>MRNQELARIFEEIGLMSEFLGDNPFRVRAYHQAARTLYDLDTPIEEIAEKGKEALMELPGVGPDLAEKILEFLRTGKVRKHEELSRKVPRGVLEVMEVPGVGPKTARLLYEGLGIDSLEKLKAALDRGDLTRLKGFGPKRAERIREGLALAQAAGKRRPLGAVLSLARSLLEAIRALPGVERAELCGSARRYKDTVGDLDFLVASREGERAVEGFVRLPQVKEVYAKGKERATVFLKNGLQVDLRVVPPESYGAGLQYLTGSKAHSIRLRALAQEKGLKLSEYGVFRGEKRIAGETEEEVYAALGLPWIPPPLREDQG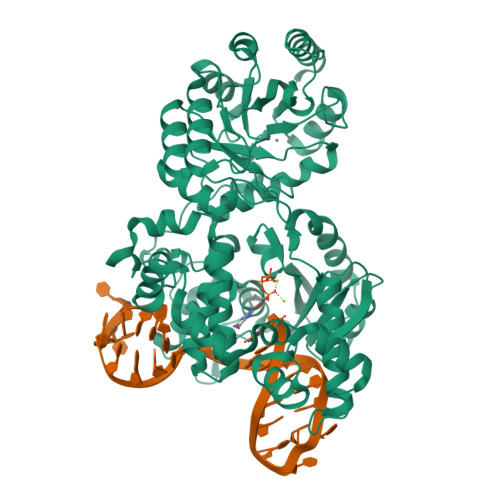EVEAALEGRLPKLLELPQVKGDLQVHSTYSDGQNTLEELWEAAKTMGYRYLAVTDHSPAVRVAGGPSPEEALKRVGEIRRFNETHGPPYLLAGAEVDIHPDGTLDYPDWVLRELDLVLVSVHSRFNLPKADQTKRLLKALENPFVHVLAHPTARLLGRRAPIEADWEAVFQKAKEKGVAVEIDGYYDRMDLPDDLARMAYGMGLWISLSTDAHQTDHLRFMELAVGTAQRAWIGPERVLNTLDYEDLLSWLKARRGV[2x]> SGKMTGIVKWFNADKGFGFITPDDGSKDVFVHFSAIQNDGYK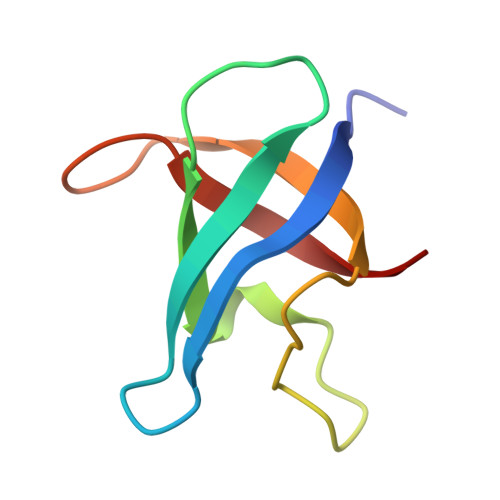SLDEGQKVSFTIESGAKGPAAGNVTSL>EQARPYAIPAGQLGDVLNRFAREAGITLSATPAQTGGYSSQGLRGSFTVQQGLARLLADTPLEAEDQGDGSFVLREAPAKDGDVLNMQAVEVFALGNNLGSTDGYLATHSQIATKTSKPLLETSQTVSVITREQIDDTASKTVQQAMRYTPGIFTGQVGASNRYDYVVMRGFADNSVDNIYLDGLKAMGDSGTFSSMQVDPYFLERIDVLKGPSSVLYGRSLPGGLVALTSKKPLYEDYRQITGSIGNMGQKEMGFDFSGPLDEEKRIAYRLIGLGKGSDTQFDHVKEERYAIAPTLAIDFSDDTTLTLQGYLQHDPNGGYHGGVPADGTLSHHNGRHISREFFDGEPSKDDFDRTQRMFGYQLEHRIDDVWSARQNFRYLDSDVDLSQVYAYGWSASEPNKLNRYFSGAREHLQAYIVDNMLQAEFATGAARHTLLTGLDYQRRRTVVDWRSGSASALDAFNPVYGDDAISYFPDDNHTRRLEQTGVYLQDLIDIDQWRFSLGLRQDWVSVTDKNRSTGSKADDDWEKFTGRIGALYLFDNGLAPYVSYSESFNPNAYSDASGTPLAPTEGKQWELGLKFQAPGSNSFYTASLFHITQENVASKEPQDNFYTSVGEVRSQGLELEAHTQLSDNLKLLGSYTYTDITYTKSLDGNQGHTPNQAPKHMASLWADYAFDAGPLSGLSIGGGARYVGETWADKENTLRVPDYTLVDARIGYDLGKLGLKGLDVSLNANNLLDKDYVASCYSLDFCYFGEKRNVTATVNYQF[2x];>[2x]DSDIKPLRMDPPVYPRMAQARGIEGRVKVLFTITSDGRIDDIQVLESVPSRMFDREVRQAMAKWRFEPRVSGGKIVARQATKMFFFKIEK

One example of siderophore piracy is the uptake of ferrioxamine B, a hydroxamate siderophore produced by many Streptomyces species, by the specific OM transporter FoxA. FoxA belongs to the family of TBDTs (transducers) and is involved in ferrioxamine B transport as well as modulation of transcriptional cascades in the bacterial cell. Here, we determined several crystal structures of FoxA from P. aeruginosa, in the apo state as well as in complex with the siderophore ferrioxamine B and TonB. Our results indicate that the transporter can exist in several different conformations, and that both substrate- and TonB-binding is required to form a translocation-competent state of the FoxA transporter in a two-step TonB-binding mechanism necessary for transport function.

In order understand the mechanism of complex formation between FoxA and TonB we determined the crystal structure of the ternary complex consisting of FoxA bound to ferrioxamine B and the C-terminal TonB domain (residues 251-340, referred to hereafter as TonBCt). Two complexes were present in the asymmetric unit, with crystal contacts generated through the exposed soluble regions of both proteins. We could resolve almost an entire FoxA molecule including the signalling domain (residues 53-820, with 11 amino acids missing from the N-terminus after the signal peptide) as well as the full TonBCt. Similar to the FhuA and BtuB-TonB complexes the primary interaction site between FoxA and TonBCt occurs through β-augmentation with parallel strands forming between residues 332-337 of TonB and residues 142-146 of FoxA. In addition to the observed β-augmentation, the unstructured polypeptide segment upstream of the TonB box (residues 135-141) forms complementary contacts with the surface of TonB molecule mediated by backbone H-bond interactions as well as side-chains Leu137, Met139 and Val142 located in a small cavity on the surface of TonB. The secondary point of contact involves the side chains of residues in the periplasmic loops and barrel interior of FoxA with several residues in the loops of TonB facing the barrel. These contacts are mediated by electrostatic forces between TonBR271 and FoxAD352, and between TonBR266 and FoxAD355 as well as a side-chain (FoxAE316) to the backbone carbonyl (TonBS300) via a hydrogen bond. In our crystal structure, the TonB fragment is located almost perpendicular to the β-barrel and the membrane plane highlighting the potentially dynamic nature of TBDR-TonB complexes, which has been suggested by recent EPR experiments. However, when ligand-loaded, FoxA association with TonBCt leads to the closure of the extracellular loops, shielding the bound siderophore inside the barrel. The inward movement of loop 8, which is seen in the ternary complex with TonBCt, places Lys657 into close proximity of the bound ferrioxamine B with its ε-amino group protruding towards the hydroxamate groups coordinating Fe3+ on the opposite side of His374.>MSASTQHRAHRWPQPLPGNDRKIWFGADYNPDQWPEDVQDEDIRLMKQAGVNIVSLAIFSWANIETSDGNFEFDWLDRVIDKLYKAGIAVDLASATASPPMWLTSAHPEVLRRDEQGHVIWPGARQHWRPTSPTFRTYALRLCREMAEHYKDNPAIVSWHVGNEYGCHNYFDYSDDAVQAFREWCRDRYGTIDKVNAAWGTNFWSQRLNSFEEILPPRYVGGEGNFTNPGRLLDFKHFCSDALKEFFCAERDVLSEVTPNIPLTTNFMVSASQNTLDYDDWAHEVDFVSNDHYFTPGSWHIDELAYSASLVDGISRKKPWFLMAQSTSAVNWREINPRKEPGELIRDSMLHLAMGADAICYFQWRQSRSGAEKFHSAMLPLAGEHSQIYRDVCALGADLDTLSDAGILRSKLSKARVAIVQDIQSEWATEHTATPTQHIREWTEPLDWFAAFANRGVTADVTPIHAQWDTYDAVVIPCVYLFSEEMAERLRTFVRNGGKAFVTYYSALADEHDRLHTEGWPGLIGDVVGVRIEEHCPLGTLFPGMLDHLDVSNGTVVHDLADVIDAIADDTTVLATFEADPATGMDGRAAITVHPYHEGGVAYIAGKLG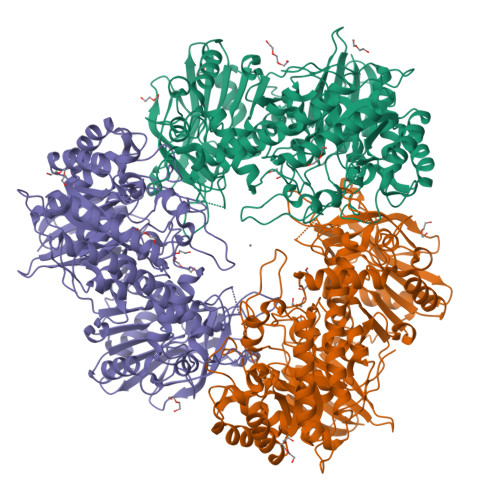RDGISQSLPEICAALGFELDADPRAGDVLRVVREQEDGAIFEFLFNRTRNTVTADRPAGDMLICSLATDSTDKVTLEPNGVLAFRR[3x]> MLRFAITLFAVITSSTCQQYGCLEGDTHKANPSPEPNMHECTLYSESSCCYANFTEQLAHSPIIKVSNSYWNRCGQLSKSCEDFTKKIECFYRCSPHAARWIDPRYTA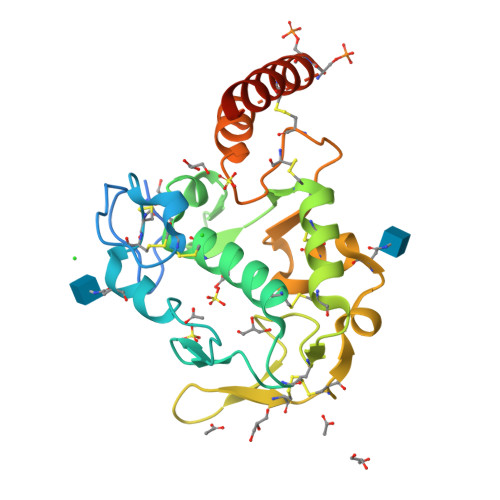AIQSVPLCQSFCDDWYEACKDDSICAHNWLTDWERDESGENHCKSKCVPYSEMYANGTDMCQSMWGESFKVSESSCLCLQMNKKDMVAIKHLLSESSEESSSMSSSEEHACQKKLLKFEALQQEEGEERR> MTFNYVIP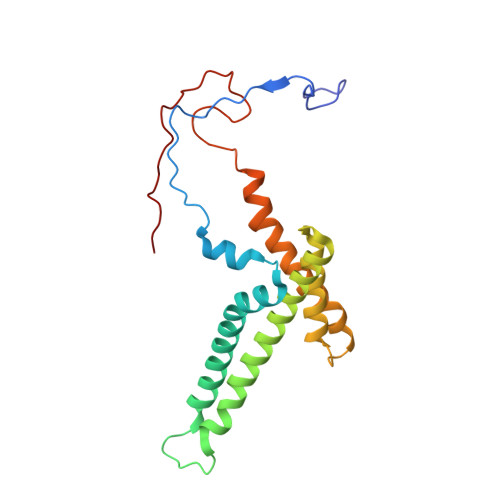YGGSSSYTINNEPVKAEEVTVDFSKEPSASSLKLADKSDWIAYTFNNVPLMATVGLLAGAHEAFLHYERTPIYGKRTYNIIKKLAPIVINKTAYATLLGAIFCATDALYENYSGKKSYTSGMVAGAATGAVFAIGRPLPQPLVWPLVFAAAPVIADLFGEVYPESMKSARGYGTPYGFENLDDAVPTRNPIRRNPHHY> STGSATTTPIDSLDDAYITPVQIGTPAQTLNLDFDTGSSDLWVFSSETTASEVDGQTIYTPSKSTTAKLLSGATWSISYGDGSSSSGDVYTDTVSVGGLTVTGQAVESAKKVSSS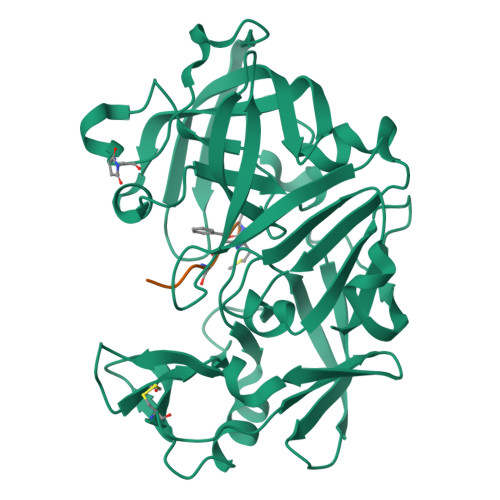FTEDSTIDGLLGLAFSTLNTVSPTQQKTFFDNAKASLDSPVFTADLGYHAPGTYNFGFIDTTAYTGSITYTAVSTKQGFWEWTSTGYAVGSGTFKSTSIDGIADTGTTLLYLPATVVSAYWAQVSGAKSSSSVGGYVFPCSATLPSFTFGVGSARIVIPGDYIDFGPISTGSSSCFGGIQSSAGIGINIFGDVALKAAFVVFNGATTPTLGFASK;> HPHLSXAH>[2x]MATERTLSIIKPDAVAKNVIGEIESRFEKAGLKIVAAKMLQLSQEQAEGFYAEHKERPFFGDLVGFMTSGPVVVQVLEGENAIAA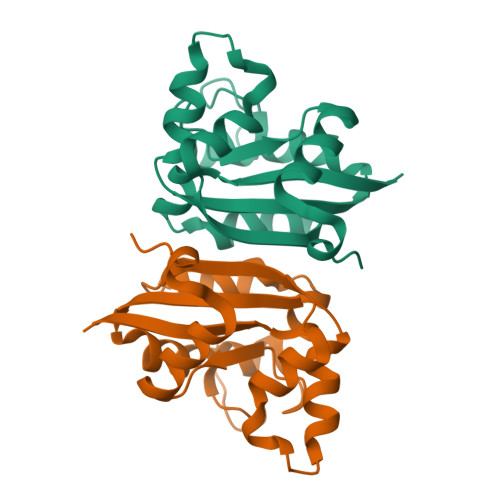NRDLMGATNPKEAEAGTIRADYAQSIDANAVHGSDSPESAAREIAYFFEESEICSR>M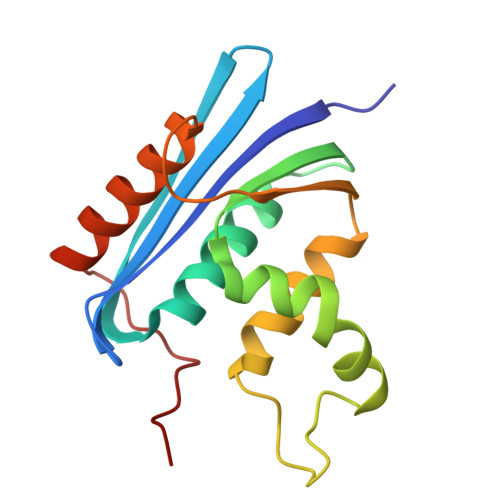LKQVEIFTDGSCLGNPGPGGYGAILRYRGREKTFSAGYTRTTNNRMELMAAIVALEALKEHCEVILSTDSQYVRQGITQWIHNWKARGWKTADKKPVKNVDLWQRLDAALGQHQIKWEWVKGAAGHPENERCDELARAAAMNPTLEDTGYQVEV[8x]>MKEKFVLIITHGDFGKGLLSGAEVIIGKQENVHTVGLNLGDNIEVVRKEVEKIIKEKLQEDKEIIIVVDL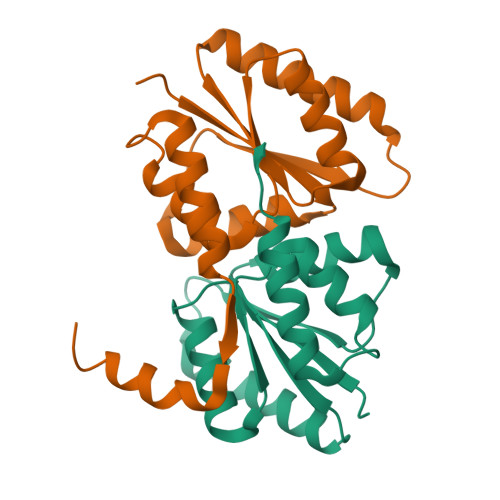FGGSPFNIALSMMKEYDVKVITGINMPMLVELLTSINVYDTTELLENISKIGKDGIKVIEKSSLKMLEHHHHHH[6x]> GSHMPPGTVDKKMVEKCWKLMDKVVRLCQNPKLALK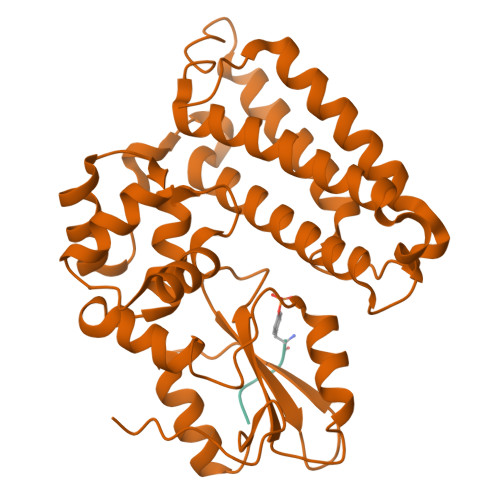NSPPYILDLLPDTYQHLRTILSRYEGKMETLGENEYFRVFMENLMKKTKQTISLFKEGKERMYEENSQPRRNLTKLSLIFSHMLAELKGIFPSGLFQGDTFRITKADAAEFWRKAFGEKTIVPWKSFRQALHEVHPISSGLEAMALKSTIDLTCNDYISVFEFDIFTRLFQPWSSLLRNWNSLAVTHPGYMAFLTYDEVKARLQKFIHKPGSYIFRLSCTRLGQWAIGYVTADGNILQTIPHNKPLFQALIDGFREGFYLFPDGRNQNPDLTG> MGYSLFPNSPKWTSKVVTYRIVSYTRDLPHITVDRLVSKALNMWGKEIPLHFRKVVWGTADIMIGFARGAHGDSYPFDGPGNTLAHAFAPGTGLGGDAHFDEDERWTDGSSLGINFLYAATHQLGHSLGMGHSSDPNAVMYPTYGNGDPQNFKLSQDDIKG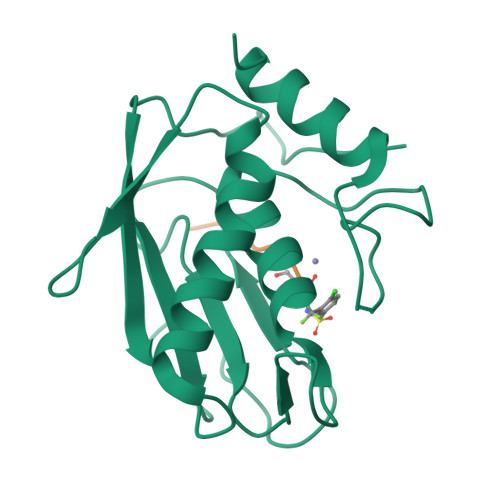IQKLYGKRSNSRKK> GLSDELEEVIVEKTKQTLASVSSGPKHTQSVPALTANETGATLPTRPSDNVETRTTYMHFNGSETDVESFLGRAACVHVTEIKNKNAAGLDNHRKEGLFNDWKINLSSLVQLRKKLELFTYVRFDSEYTILATASQPEASSYSSNLTVQAMYVPPGAPNPKEWDDYTWQSASNPSVFFKVGETSRFSVPFVGIASAYNCFYDGYSHDDPDTPYGITVLNHMGSMAFRVVNEHDVHTTIVKIRVYHRAKHVEAWIPRAPRALPYVSIGRTNYPRDSKTIVKKRTNIKTY;> SPNVEACGYSDRVQQITLGNSTITTQEARNAIVCYAEWPEYLSDNDASDVNKTSKPDISVCRFYTLDSKTWKATSKGWCWKLPDALKDMGVFGQNMFYHSLGRTGYTIHVQCNATKFHSGCLLVVVIPEHQLASHEGGTVSVKYKYTHPGDRGIDLDTVEVAGGPTSDAIYNMDGTLLGNLLIFPHQFINMRTNNTATIVVPYINSVPIDSMTRHN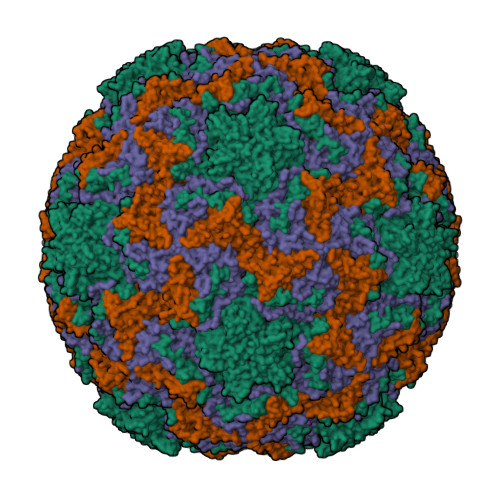NVSLMVVPIAPLNAPTGSSPTLPVTVTIAPMCTEFTGIRSRSIVPQ;> GLPTTTLPGSGQFLTTDDRQSPSALPSYEPTPRIHIPGKVRNLLEIIQVGTLIPMNNTGTNDNVTNYLIPLHADRQNEQIFGTKLYIGDGVFKTTLLGEIAQYYTHWSGSLRISLMYTGPALSSAKIILAYTPPGTRGPEDKKEAMLGTHVVWDIGLQSTIVMTIPWTSGVQFRYTDPDTYTSAGYLSCWYLTSLILPPQTSGQVYLLSFISACPDFKLRLMKDTQTISQTDALTE;> GAQVSTQKSGSHENQNILTNGSNQTYTVINYYKDAASSSSAGQSFSMDPSKFTEPVKDLMLKGAPALN> MNRVQSGFRVPARVLNSLAHLQDGLNIFMDPDWRQIRHVDDWALAITMESAELIDSYPWKWWKNVKAQTDMHNVRIEIADILHFSLSGEIQKRTQDEKGADDVALKSLKEMGFF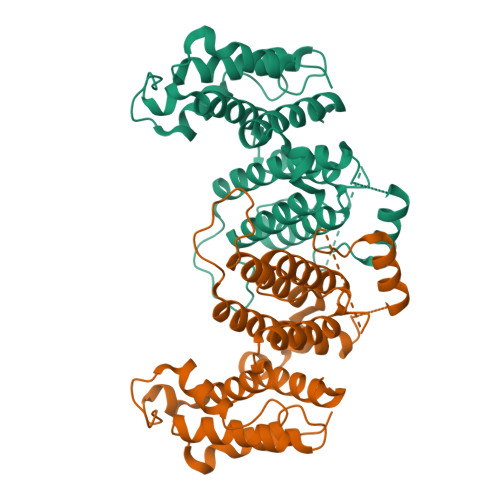CRPPAHAKSTAASGQRTNGGDGDGDDELLELMFFPLTEVASAVATFRNIIQLASIYRFDLITKGLLLAAQDLDFNLVGYYVAKYTLNQIRQLKGYKEGVYVKVREGVEDNELLHECVQSVSVEDVLNEGTYLKAWEKIACSVFDAFGMPEEERRHAYDWLKSAALDGKG>IVGGYTCEENSLPYQVSLNSGSHFCGGSLISEQWVVSAAHCYKTRIQVRLGEHNIKVLEGNEQFINAAKIIRHPKYNRDTLDNDIMLIKLSSPAVINARVSTISLPTAPPAAGTECLISGWGNTLSFGADYPDELKCLDAPVLTQAECKASYPGKITNSMFCVGFLEGGK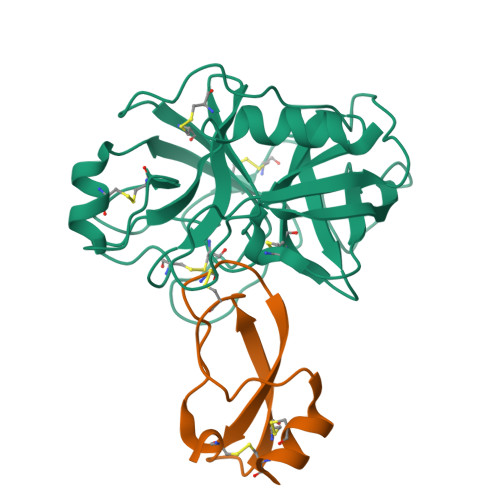DSCQRDAGGPVVCNGQLQGVVSWGHGCAWKNRPGVYTKVYNYVDWIKDTIAANS[2x];>[2x]YVDYKDDDDKEFEVCSEQAETGPCRAGFSRWYFDVTEGKCAPFVYGGCGGNRNNFDTEEYCMAVCGSAIPRHHHHHHAAAN> MHHHHHHASENLYFQGAMGVEVCVKAAVGHPDTLGDSPFSQRVLLTLEEKKVPYEMKLIDVQNKPDWFLKISPEGKVPVFNGG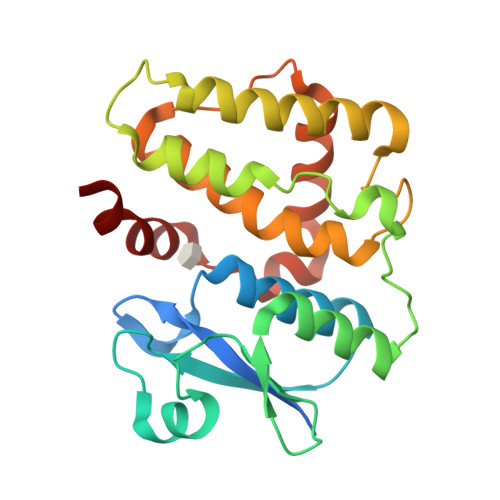DGKWIPDSDVITQVIEEKYPTPSLVTPPEYASVGSKIFSCFTTFLKSKDPNDGSEKALLTELQALEEHLKAHGPFINGQNISAADLSLAPKLYHLQVALEHFKGWKIPEDLTNVHAYTEALFSRESFIKTKAAKEHLIAGWAPKVNA>[2x]MNITQAAEQAIRLWFNTPDPMQRLHMAKTIRTWIRQDKFAQVDQANMPNCVQQILNIIYDGLKPQPVQLPISYYAQLWYNLLDILRRFTFLPIISPYIHQVVQMFCPRENGPQDFRELICNLISLNWQKDPHMKHCANQVFQIFNCIIMGVKNEKLRTEFAQHLKFEKLVGTLSEYFNPQVHPGMINPAIFIIFRFIISKDTRLKDYFIWNNNPHDQPPPPTGLIIKLNAVMIGSYRLIAGQNPETLPQNPELAHLIQVIIRTFDLLGLLLHDSDAIDGFVRSDGVGAITTVVQYPNNDLIRAGCKLLLQVSDAKALAKTPLENILPFLLRLIEIHPD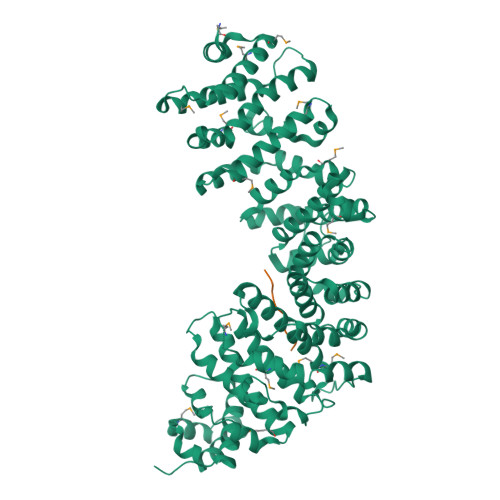DEVIYSGTGFLSNVVAHKQHVKDIAIRSNAIFLLHTIISKYPRLDELTDAPKRNRVCEIICNCLRTLNNFLMMWIPTPNGETKTAGPNEKQQVCKFIEIDILKKLMSCLSCEGMDTPGLLELRSTILRSFILLLRTPFVPKDGVLNVIDENRKENLIGHICAAYSWVFRQPNNTRTQSTKQQLVERTISLLLVLMEQCGAEKEVAQYSYSIDCPLNLLNGNQVKPTFIHNVLVVCDKILEHCPTRADIWTIDRPMLEGLTNHRNSDIAKAANSLLSRFPEN;>GDEVKVFR[2x]> GCCCGGAUAGCUCAGUCGGUAGAGCAGCGGAGCUGUUAGUCUACGUGGACCGACAAAGACAGAUUCUUUGAGGGAGCUAAGCUCAACGUAGUUCUAACAGCUCCGCGGGUCCAGGGUUCAAGUCCCUGUUCGGGCGCCA

Flaviviruses use a ~70 nucleotide stem-loop structure called stem-loop A (SLA) at the 5′ end of the RNA genome as a promoter for RNA synthesis. Flaviviral polymerase NS5 specifically recognizes SLA to initiate RNA synthesis and methylate the 5′ guanosine cap. Here we report crystal structures of flavivirus SLA; DENV and ZIKV SLA were determined to 3.4 and 3.8 Å resolution, respectively. Both structures show similar structural elements, consisting of a top stem-loop, a side loop, and a bottom stem, but differ in size and the relative arrangements of the individual elements.

The SLA structures were determined using a chimeric RNA, wherein the DENV2 SLA (nucleotides 1–70) or ZIKV SLA (nucleotides 1–71) was inserted into the anticodon loop of human tRNALys (tRNA-SLADENV and tRNA-SLAZIKV). DENV SLA is a 65 Å long by 50 Å wide, ‘L’-shaped molecule, consisting of a top stem-loop (9 bp), a side loop (9 nt), and a bottom stem (16 bp). The top stem-loop is roughly perpendicular to the bottom stem, which extends from the tRNA moiety. When compared to the predicted secondary structure, the structure of DENV SLA has two major differences near the critical 3-way junction, where the top stem-loop, side loop and the bottom stem meet. First, the predicted bulge (17GGA19) between the top and bottom stem does not exist. Instead, the 18GA19 form Watson-Crick base pairs with the 53UC54 that was predicted to be in the side stem, resulting in the bottom stem being extended by 3 base pairs compared to the prediction. Thus, the predicted side stem becomes a single-stranded side loop. Surprisingly, the side loop reveals the previously undetected self-complementary sequence (46GCUAAGC52) that forms intermolecular Watson-Crick base pairs with the equivalent region from the second SLA molecule in palindromic order with one mismatch. The two SLA molecules form a continuous helical stack from the bottom stem of one SLA molecule, through the kissing loop, to the bottom stem of the second SLA molecule. The side loop-side loop helix is further stabilized by π-π stacking interactions between two 45A bases in the dimer. As a consequence of these interactions, DENV SLA dimer has a unique intermolecular three-way (3-way) junction structure, where one helix of the 3-way junction is shared between the two SLA molecules.>[2x]MSRNSLDLYEEILTEEGTAKEATYNDLQVEYGKAQLQMKELMKKFKEIQAQNFSLI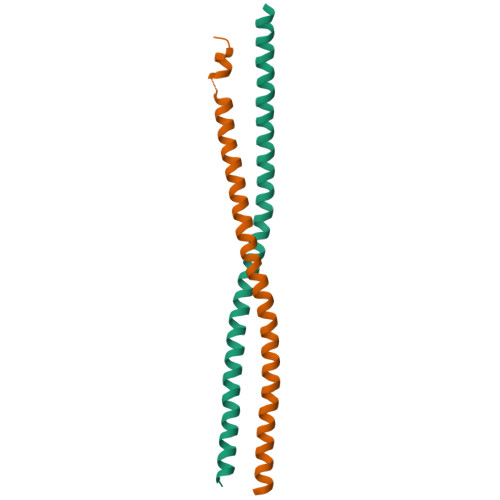NENQSLKKNISALIKTARVEINRKDEEISNLHLEHHHHHH In this study, we designed a novel L-amino acid oxidase, HTAncLAAO2, by ancestral sequence reconstruction, exhibiting high thermostability and long-term stability. L-amino acid deaminase (LAADs)16,17,19–23 and L-amino acid oxidases (LAAOs)15,24–27 are key biocatalysts efficiently converting L-AAs to keto acids. An advantage of LAAOs is that the enzyme only requires O2 molecules to regenerate oxidized FAD. HTAncLAAO2 demonstrated substrate selectivity almost identical to, and higher activity than, the HTAncLAAO27; these properties make the enzyme suitable for synthesizing D-AAs from L- or rac-AAs.

The overall structure of HTAncLAAO2, determined at a 2.2 Å resolution, indicating that the enzyme has typical folding of amine oxidase superfamily, such as L-Lysine α-oxidase and LAAO from Pseudoalteromonas species, in spite that they shared low sequence identity to each other. The unique point of HTAncLAAO2 is that the enzyme displays a distinctive octameric state. We performed gel-filtration and negative-stained EM analyses to investigate the oligomeric state in physiological conditions. Gel-filtration chromatography analysis suggested that the HTAncLAAO2 eluted as 544 kDa (denoted by the red star in Fig. 1B), indicating that the formation of complexes in solution by eight HTAncLAAO2 molecules, each with a molecular weight of 63 kDa. The results show that HTAncLAAO2 has an octameric, ninja-star-like structure. This distinctive oligomeric state may be origin for the high thermostability and long-term stability of HTAncLAAOs; other thermostable enzymes also had an oligomeric form to improve the stability. Alterations in the structure to better recognize other L-AAs could potentially enhance HTAncLAAO2’s activity towards substrates that currently show weak activity. The thermostability (red colored in Fig. 2C) and long-term stability (red colored in Fig. 2D) of HTAncLAAO2, measured using L-Met as a substrate, were similar to those of HTAncLAAO; a T1/2 of about 85 °C, and residual activity exceeding 95% following a 7-day incubation at 30 °C. We unexpectedly found a NOS bridge between residues K304 and C505 which are located remotely from the active site. In conclusion, the NOS bridge identified in HTAncLAAO2 had minimal influence on in vitro parameters such as enzyme activity and thermostability. Alternatively, we predicted L-Trp binding form of HTAncLAAO2 by superposing the L-Trp binding structure of AncLAAO-N4 based on FAD molecule. The HTAncLAAO2 structure suggested that the side chains of five hydrophobic residues (W220, Y383, W482, and W520 depicted in Fig. 4B, and L320 in Fig. S3) were located proximal to the indole group of L-Trp. Enzyme kinetic analysis suggested that Tte W220A mutation likely introduces a cavity in the active site, accommodating the long-chain L-AAs while compromising affinity for L-Phe, L-Leu, L-Met, and L-Ile.

>[4x]MENEKIDIAIVGGGVSGVYSAWKLKTKYPNKKIVLFEGGDHIGGRLLSVIPPGIPNMVAELGGMRILENTQKLIVKLIDDINEKLSQEDQIELYDFPVDQPQNIAYLRGEHLRLFDFTNDPDKVPYKLSFLEKGNTSGTIIVNAIEQLVPGITNTDLTEEERLKMCQEATFEGAPLYTLGFWNLLYRVISGEAYQFSIDSGGYNSTLVNWNAADAIPWYLSDFGIKPVYKGFKNGFQQVPISLANFFEEDGGEIRLNAKLEGFEFKNNLFELTIDGEIIEATQLILAMPRRSLDLLTNTSPKLQEIQSLIGSVTPRPLFKVFTTYSSPWWRNAGYTDSEGGYIPLQSGRTVTDLPIRQTYYWPKNNGQPSVSGESMLLASYDDGSNIGFWDGLRPQRKKAWKKGLSHAELADDPFIGEYSETESLLSKALNQTWHQYKAPRKMVEELSRQLKQIHDVDYTPAVKNASFRDWGEDPFGGGWNSWNIGVKSWEVKEKIVHPIDNCSLYICGEAYSDGQGWVEGALQTADIMLKKFIAVESKTSVKEEAILEHHHHHH2,5-dihydroxybenzenesulfonic acid | C6 H6 O5 S | 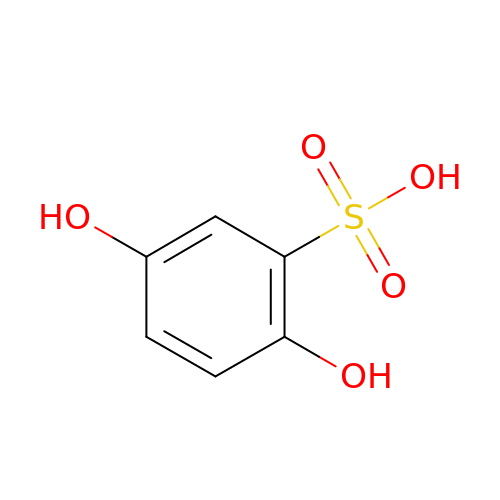IKQCSJBQLWJEPU-UHFFFAOYSA-N> AYTTFSQTKNDQLKEPMFFGQPVNVARYDQQKYDIFEKLIEKQLSFFWRPEEVDVSRDRIDYQALPEHEKHIFISNLKYQTLLDSIQGRSPNVALLPLISIPE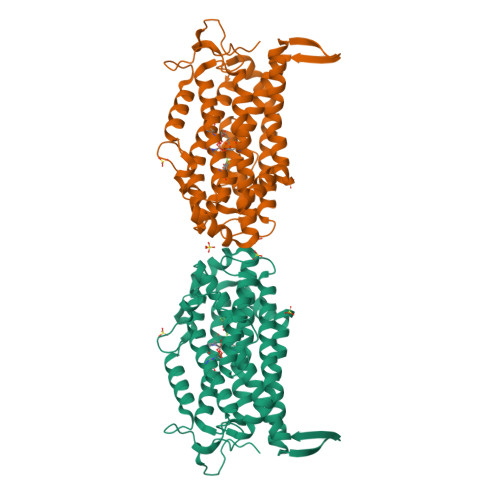LETWVETWAFSETIHSRSXTHIIRNIVNDPSVVFDDIVTNEQIQKRAEGISSYYDELIEMTSYWHLLGEGTHTVNGKTVTVSLRELKKKLYLCLMSVNALEAIRFYVSFACSFAFAERELMEGNAKIIRLIARDEALHLTGTQHMLNLLRSGADDPEMAEIAEECKQECYDLFVQAAQQEKDWADYLFRDGSMIGLNKDILCQYVEYITNIRMQAVGLDLPFQTRSNPIPWINTWLVSDNVQVAPQEVEVSSYLVGQIDSEVDTDDLSNFQL UdgX excises uracil from uracil-containing DNA to concurrently form a covalent bond with the resulting AP-DNA. Structurally, UdgX is highly similar to family-4 UDGs (F4-UDGs). However, UdgX is unique in possessing a flexible R-loop (105KRRIH109). Our earlier studies allowed us to propose a reaction mechanism of UdgX, which involves the formation of a covalent bond between H109 of UdgX with the C1′ position of the target deoxyribose sugar concurrently with the uracil excision from this site in DNA.

Substitutions of His109 in MsmUdgX with Ser, Gly, Ala, Gln, Cys and Lys showed the loss of its covalent complex formation with DNA but gained canonical UDG activities. However, H109 substitutions by Gln or Lys, showed poor activity. Both Cys and Ala mutations of H109 showed intermediate Kcat/Km values. However, to better understand the mechanism of uracil excision by the H109 mutants, we determined their structures along with a pentameric DNA, TTUTT by X-ray crystallography. The DNA backbone could not be modelled into the experimental electron density map in any of the mutant structures that were determined. Nonetheless, all structures revealed the excised uracil and the side chain substitutions at position 109. The structures also revealed invariant interactions of N91 and H178 with uracil. When we arranged the mutants in the order of increasing cavity sizes (left), we noted that the canonical UDG activity of the mutants increased with their increasing cavity sizes to begin with and then with a further increase in the cavity size, the UDG activity declined (right). It suggested that the initial increase in UDG activity (H109K to H109Q to H109G) occurred because of the efficiency with which the water molecule could be localized to make a nucleophilic attack on the C1′ position. However, a further increase in the cavity size (H109S to H109C to H109A) perhaps destabilizes the bound water, thereby decreasing the UDG activity.

> GAQDFVPHTADLAELAAAAGECRGCGLYRDATQAVFGAGGRSARIMMIGEQPGDKEDLAGLPFVGPAGRLLDRALEAADIDRDALYVTNAVKHFKFTRAAGGKRRICKTPSRTEVVACRPWLIAEMTSVEPDVVVLLGATAAKALLGNDFRVTQHRGEVLHVDDVPGDPALVATVHPSSLLRGPKEERESAFAGLVDDLRVAADV> PIVVQAAGGRSWKAVDSVMFQQLQTVAMQHGLVSEDFERQLAYYATTWTSKDILEVLAMMPGNRAQKELIQGKLNEEAERWRRNNPPPPAGGGLTVDQIMGVGQTNQAAAQA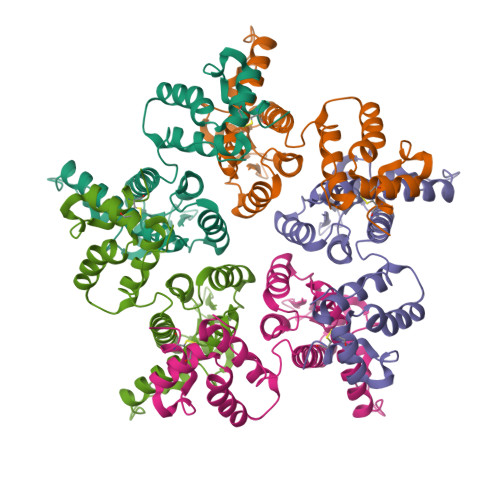NMDQARQICLQWVINALRAVRHMAHRPGNPMLVKQKTNEPYEDFAARLLEAIDAEPVTQPIKDYLKLTLSYTNASADCQKQMDRTLGQRVQQASVEEKMQACRDVGSEGFHHHHHH> IIANAVVAQDGTGDYQTLAEAVAAAPDKSKTRYVIYVKRGTYKENVEVASNKMNLMIVGDGMYATTITGSLNVVDGSTTFRSATLAAVGQGFILQDICIQNTAGPAKDQAVALRVGADMSVINRCRIDAYQDTLYAHSQRQFYRDSYVTGTVDFIFGNAAVVFQKCQLVARKPGKYQQNMVTAQGRTDPNQ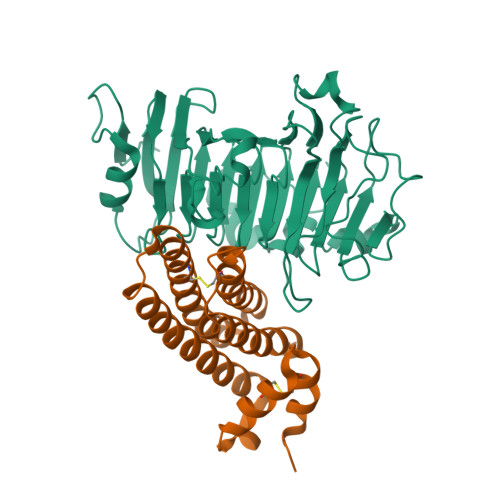ATGTSIQFCNIIASSDLEPVLKEFPTYLGRPWKEYSRTVVMESYLGGLINPAGWAEWDGDFALKTLYYGEFMNNGPGAGTSKRVKWPGYHVITDPAKAMPFTVAKLIQGGSWLRSTGVAYVDGLYD;> FENHLISEICPKTRNPSLCLQALESDPRSASKDLKGLGQFSIDIAQASAKQTSKIIASLTNQATDPKLKGRYETCSENYADAIDSLGQAKQFLTSGDYNSLNIYASAAFDGAGTCEDSFEGPPNIPTQLHQADLKLEDLCDIVLVISNLLPGS> SMTSSANEDMPVERILEAELAVEPKTETYVEANMGLNPSSPNDPVTNICQAADKQLFTLVEWAKRIPHFSELPLDDQVILLRAGWNELLIASFSHRSIAVKDGILLATGLHVHRNSAHSAGVGAIFDRVLTELVSKMRDMQMDKTELGCLRAIVLFNPDSKGLSNPAEVEALREKVYASLEAYCKHKYPEQPGRFAKLLLRLPALRSIGLKCLEHLFFFKLIGDTPIDTFLMEMLEAPHQMT;> KHKILHRLLQDSSY

The nuclear retinoid X receptor (RXR) is a unique family of ligand-activated transcription factors, which in humans comprises of three members, namely, RXRα (NR2B1), RXRβ (NR2B2) and RXRγ (NR2B3). All three RXR isoforms typically function as a universal heterodimer partner for other nuclear receptors, including the type II thyroid hormone receptors (THRs, NR1A1-2) and the peroxisome proliferator-activated receptors (PPARs, NR1C1-3). Here, we report a complete set of the crystal structures for all three RXR isoforms in active, ligand-bound conformation with an identical ligand. In addition, we discovered saturated fatty acids, including palmitic acid (PA), myristic acid (MA) and stearic acid (SA), as RXR modulators capable of inducing the recruitment of co-regulators to the RXR ligand-binding domain (LBD) and hence, activating the receptor.

Upon crystallization and structure determination of the recombinant RXRα LBD in complex with the glucocorticoid receptor interacting protein 1 (GRIP-1) co-regulator peptide, we unexpectedly observed extra electron density within the ligand-binding pocket of the protein. Based on the shape of the density, we hypothesized the presence of a fatty acid, likely contaminated from the recombinant protein production in Escherichia coli. Mass spectrometric analysis further confirmed the identity of this ligand as palmitic acid (PA), a widely abundant fatty acid in bacteria and eukaryotic cells, which was successfully modelled in the crystal structure. A structural comparison with other known RXRα ligands, such as JP175 (compound 24), revealed that PA occupied the orthosteric binding pocket typically targeted by other small molecule modulators and the accommodation of this fatty acid did not require any structural alterations (see Section 2.3). The carboxylic acid moiety of the fatty acid formed a salt-bridge contact with the highly conserved Arg316 (using the numbering of RXRα as an example), a canonical interaction typically observed for most RXR ligands. The saturated hydrocarbon tail was seen to elongate along the hydrophobic groove until C11-C12 where an ~90° bend was formed to ascend the rest of the tail toward the hydrophobic pocket created by Phe346 and Leu324. In comparison with RXR synthetic small molecule modulators, such as JP175 (compound 24), this L-shape conformation allowed the fatty acid to fully occupy the vast hydrophobic space of the ligand-binding pocket without the need for structural rearrangement of the lining residues. Thus, this RXRα-PA-GRIP-1 tertiary complex opens the possibility of involvement of fatty acids in RXR signaling. We observed indeed that all three saturated fatty acids promoted SRC-1 recruitment to RXRα, with an increase in their efficacies seemingly corresponding to longer chain lengths (EC50 of 3.2 µM for MA, 6.6 µM for PA and 19 µM for SA).Here, we present the discovery of a promiscuous allosteric site in SMYD2, a unique member of the protein lysine methyltransferase family characterized by the co-presence of the SET and MYND domains. SMYD2 is a critical regulator of numerous cellular processes, methylating both histone and non-histone proteins to control chromatin remodeling, DNA damage response, cell cycle progression, cell differentiation, cell survival, and inflammation. We have determined four crystal structures of SMYD2, including a wild-type protein structure in complex with a PARP1 peptide, a wild-type protein structure in complex with an ethylene glycol polymer (PEG), and two structures of SMYD2 mutants. In all structures, SMYD2 maintains a bilobal fold, with the N- and C-lobes displaying a similar orientation and a similar degree of opening.

Two peptide binding sites are identified in the wild-type SMYD2 structure in complex with a Lys528-containing PARP1 peptide. One corresponds to the well-known substrate binding site, and the other is new and had not been characterized before. At the substrate binding site, the PARP1 peptide binds in a U-shaped conformation, sandwiched by the β8–β9 hairpin from the SET domain and a loop connecting the SET and post-SET domains. The target lysine (Lys528) is located at the U-base of the peptide, with its side chain inserted into the target lysine access channel. In this position, the epsilon nitrogen of Lys528 is adjacent to AdoHcy at the cofactor binding site. The novel secondary binding site is located near the substrate binding site in the cleft between the N- and C-lobes. Two subsites were defined based on their interactions with the peptide: the M-subsite interacts with Met-5 of the peptide, while the L-subsite interacts with Leu-3. Key residues for peptide binding at the M-subsite include Leu351, Lys387, Arg390, and Leu391, which form a shallow hydrophobic pocket where Met-5 is bound. At the L-subsite, Trp356 is important for peptide binding, as Leu-3 is stacked between the side chain of this residue and the main chains of Arg390 and Gly394. Based on this analysis, we conclude that SMYD2 binds to two individual PARP1 peptides in the structure.

>[2x]MRAEGLGGLERFCSPGKGRGLRALQPFQVGDLLFSCPAYAYVLTVNERGNHCEYCFTRKEGLSKCGRCKQAFYCNVECQKEDWPMHKLECSPMVVFGENWNPSETVRLTARILAKQKIHPERTPSEKLLAVKEFESHLDKLDNEKKDLIQSDIAALHHFYSKHLEFPDNDSLVVLFAQVNCNGFTIEDEELSHLGSAIFPDVALMNHSCCPNVIVTYKGTLAEVRAVQEIKPGEEVFTSYIDLLYPTEDRNDRLRDSYFFTCECQECTTKDKDKAKVEIRKLSDPPKAEAIRDMVRYARNVIEEFRRAKHYKSPSELLEICELSQEKMSSVFEDSNVYMLHMMYQAMGVCLYMQDWEGALQYGQKIIKPYSKHYPLYSLNVASMWLKLGRLYMGLEHKAAGEKALKKAIAIMEVAHGKDHPYISEIKQEIESH;>[4x]RMKLTLKGGAAVD> ADNLAEFHVQNQECDSCHTPDGELSNDSLTYENTQCVSCHGTLAEVAETTKHEHYNAHASHFPGEVACTSCHSAHEKSMVYCDSCHSFDFNMPYAKKWLRDEPTIAELAKDKSERQAALASAPHDTVDVVVVGSGGAGFSAAISATDSGAKVILIEKEPVIGGNAKLAAGGMNAAWTDQQKAKKITDSPELMFEDTMKGGQNINDPALVKVLSSHSKDSVDWMTAMGADLTDVGMMGGASVNRAHRPTGGAGVGAHVVQVLYDNAVKRNIDLRMNTRGIEVLKDDKGTVKGILVKGMYKGYYWVKADAVILATGGFAKNNERVAKLDPSLKGFISTNQPGAVGDGLDVAENAGGALKDMQYIQAHPTLSVKGGVMVTEAVKGNGAILVNREGKRFVNEITTRDKASAAILAQTGKSAYLIFDDSVRKSLSKIDKYIGLGVAPTADSLVKLGKMEGIDGKALTETVARYNSLVSSGKDTDFERPNLPRALNEGNYYAIEVTPGVHHTMGGVMIDTK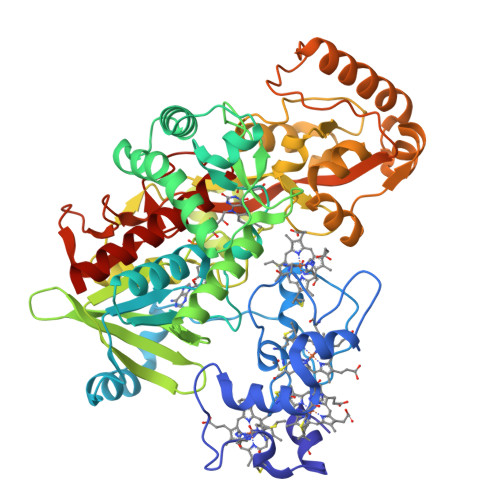AEVMNAKKQVIPGLYGAGEVTGGVHGANRLGGNAISDIITFGRLAGEEAAKYSKKN> XSLSATDKARVKALWDKIEG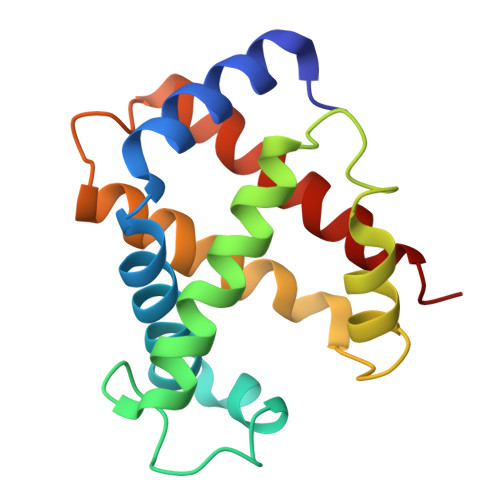KSAELGAEALGRMLVSFPQTKIYFSEWGQDLGPQTPQVRNHGAVIMAAVGKAVKSIDNLVGGLSQLSELHAFKLRVDPANFKILAHNIILVISMYFPGDFTPEVHLSVDKFLACLALALSEKYR> XVTIDADLMDAADLLEGEQVTIVDI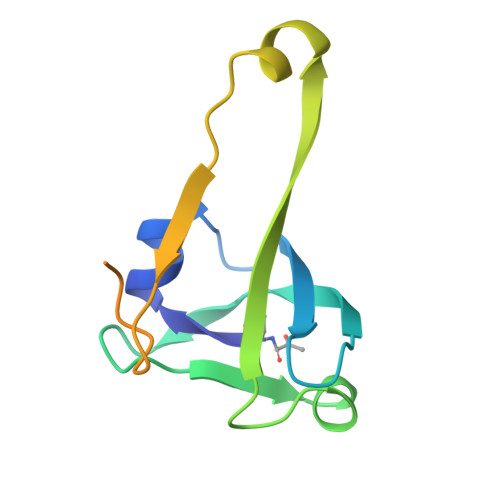DNGARLVTYAITGERGSGVIGINGAAAHLVHPGDLVILIAYATMDDARARTYQPRIVFVDAYNKPIDMGHDPAFVPENAGELLDPRLGVGLEHHHHHH5-amino-1-pyridin-3-ylpentan-1-one | 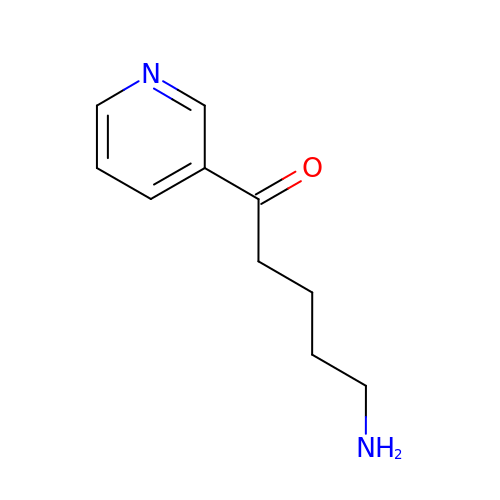C10 H14 N2 O | GSEJHUSUJYZWBW-UHFFFAOYSA-N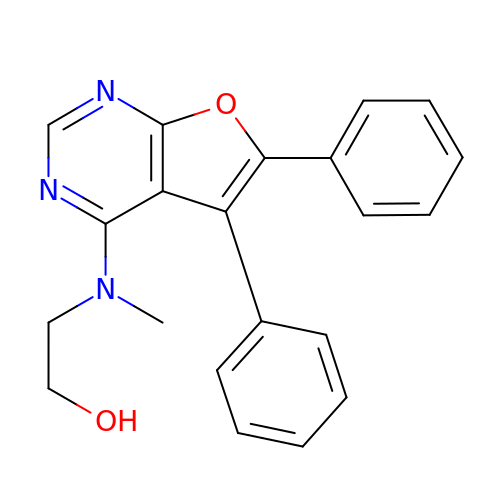(5,6-DIPHENYL-FURO[2,3-D]PYRIMIDIN-4-YLAMINO)-ACETIC | C21 H19 N3 O2 | VDJWWYRYKMXMKA-UHFFFAOYSA-N1,3,3-TRIMETHYL-2-OXABICYCLO[2.2.2]OCTANE | C10 H18 O | 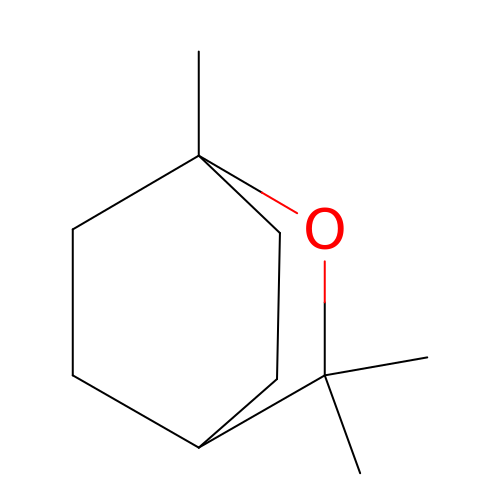WEEGYLXZBRQIMU-WAAGHKOSSA-N> MSLNTEIEMNELLEKAKKIKCLICDVDGVLSDGLLHIDNHGNELKSFHVQDGMGLKLLMAAGIQVAIITTAQNAVVDHRMEQLGITHYYKGQVDKRSAYQHLKKTL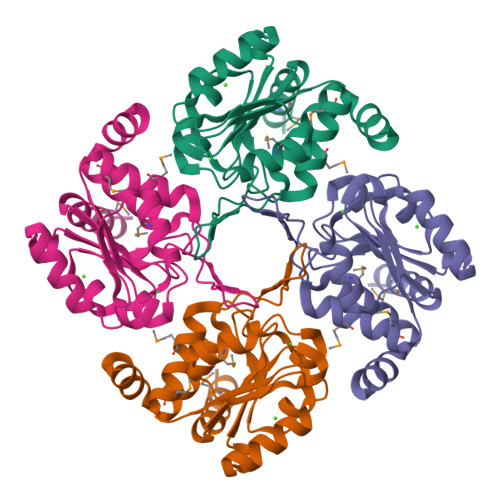GLNDDEFAYIGDDLPDLPLIQQVGLGVAVSNAVPQVLEFADWRTERTGGRGAVRELCDLILNAQNKAELAITGYLKQEGHHHHHH> AKMMQREITKTTVNVAKMVMVDGEVQVEQLPSETFVGNLT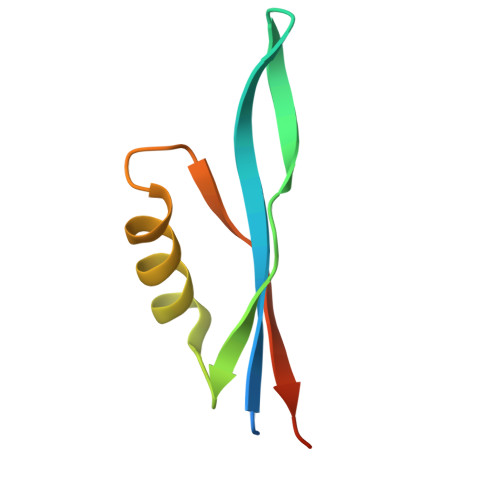MEQAQWRMKRKYKGEPVQVVSVEPNTEVYELP> LVTLVF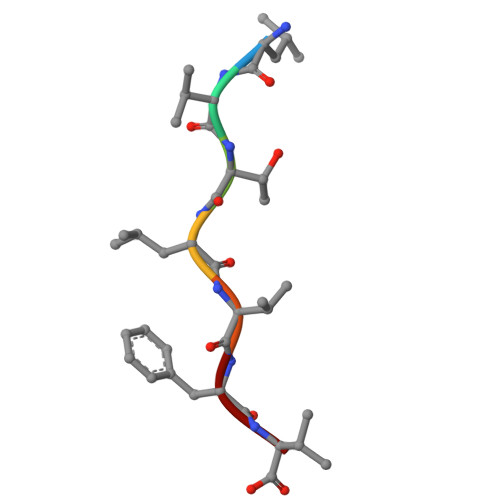V The sliding clamp is a ring-shaped protein complex that encircles DNA with the help of clamp loader in an ATP-dependent manner, and slides along the DNA. In prokaryotes, however, β-clamp is a homodimer, with each monomer consisting of three globular domains, and in this way β-clamp displays a six-domain ring. Although β-clamp is part of the DNA polymerase III holoenzyme, it is not attached to polymerase III permanently like the other subunits. β-clamp is loaded on the DNA, by clamp loader, a subunit of DNA Pol III. In both prokaryotes and eukaryotes, a key feature of this clamp-binding motif is the presence of hydrophobic amino acid residues that bind to the hydrophobic pocket in the C-terminal region of the clamp.

In the space group P2 two monomers were present per asymmetric unit. However there is no significant difference observed between these two structures from different space groups, the structural alignment of both yielded an RMSD of 0.15 Å. As expected for a prokaryotic β-clamp, each monomeric unit of Hpβ-clamp consists of three domains. In Hpβ-clamp, domains I, II, and III were observed to span residues Met1to Phe118, Pro119 to Pro 250, and Lys251 to Leu374, respectively. Domain I comprised of nine antiparallel β-strands and two alpha helices, domain II having eight β-strands and two alpha helices, and domain III with eight β-strands and two helices. As seen in β-clamp from other organisms, Hpβ-clamp form a head-to-tail dimer, i.e., the N-terminus of one monomer interacting with the C-terminus of another monomer. Two salt bridges are formed between Glu266 and Glu298 of chain A with Lys83 and Lys74 of chain B, and another set of equivalent salt bridges also formed between Glu 266 of chain B and Lys 83 of chain A, and between Glu 298 of chain B and Lys 74 of chain A. These salt bridges and several hydrophobic interactions were observed to mediate the association between the monomers. Perhaps most notably, two major DNA-interacting loops of β-clamp were observed to adopt quite different conformations in H. pylori compared to the β-clamp in E. coli and the other organisms. The loop spanning residues 20 to 28 from domain I was found to be oriented in an opposite direction in the Hpβ-clamp structure compared to the corresponding loop in the clamp structures of other organisms. Despite the oppositely oriented loops, our superposition of Hpβ-clamp with DNA-bound Ecβ-clamp showed the side chain of Hpβ-clamp Lys23 (which corresponds to Arg 24 Ecβ-clamp) still to be in a position close to DNA, suggesting that Lys23 of Hpβ-clamp may participate in DNA binding and may be crucial for binding to DNA.

>[2x]MAMKISVSKNDLENALRYLQAFLDKKDASSIASHIHLEVIKEKLFLKASDSDIGLKSYIFTQSSDKEGVGTINGKKFLDIISCLKDSNIILETKDDSLAIKQNKSSFKLPMFDADEFPEFPVIDPKVSIEVNAPFLVDAFKKIAPVIEQTSHKRELAGILMQFDQKHQTLSVVGTDTKRLSYTQLEKISIHSTEEDISCILPKRALLEILKLFYENFSFKSDGMLAVIENEMHTFFTKLIDGNYPDYQKILPKEYISSFTLGKEEFKESIKLCSSLSSTIKLTLEKNNALFESLDSEHSETAKTSVEIEKGLDIEKAFHLGVNAKFFLEALNALGTTQFVLRCNEPSSPFLIQESLDEKQSHLNAKISTLMMPITLELHHHHHH>[2x]AGQQQPLPVPPLLESRRGQPLFMTVQRAHWSFTPGTRASVWGINGRYLGPTIRVWKGDDVKLIYSNRLTENVSMTVAGLQVPGPLMGGPARMMSPNADWAPVLPIRQNAATLWYHANTPNRTAQQVYNGLAGMWLVEDEVSKSLPIPNHYGVDDFPVIIQDKRLDNFGTPEYNEPGSGGFVGDTLLVNGVQSPYVEVSRGWVRLRLLNASNSRRYQLQMNDGRPLHVISGDQGFLPAPVSVKQLSLAPGERREILVDMSNGDEVSITCGEAASIVDRIRGFFEPSSILVSTLVLTLRPTGLLPLVTDSLPMRLLPTEIMAGSPIRSRDISLGDDPGINGQLWDVNRIDVTAQQGTWERWTVRADEPQAFHIEGVMFQIRNVNGAMPFPEDRGWKDTVWVDGQVELLVYFGQPSWAHFPFYFNSQTLEMADRGSIGQLLVNPVPRSHHHHHH

SufI is a water-soluble, periplasmic protein. The sequence of SufI shows that it is a member of the multicopper oxidase superfamily. The overall structure of SufI is very similar to that of CueO and contains three cupredoxin-like domains. Indeed, access to the region of the structure that forms the active site in multicopper oxidases is blocked in SufI by highly conserved residues. Together, these observations suggest that SufI is neither a copper-binding protein nor an enzyme.

The two molecules of each asymmetric unit are essentially the same within experimental error (rmsds over 408 and 406 Cα atoms of 1.1 and 0.9 Å for the orthorhombic and monoclinic crystals, respectively). Of the two data sets, the orthorhombic crystals diffracted to higher resolution (1.9 Å compared to 2.6 Å). The structure of SufI, determined here at a resolution of 1.9 Å by X-ray crystallography, confirms that the protein belongs to the multicopper oxidase family. No electron density was observed for the hexahistidine affinity tag, with the exception of the arginine residue of the affinity tag linker in chain A of the orthorhombic structure. The main areas of difference between the two crystal forms lie between residues 42–47, 55–66 and 326–334. Residues 42–47 are found in a loop that leads into the first domain, while residues 326–334 compose the long linker between domains 2 and 3. The electron density for both of these regions was poor and often missing entirely for the side chains. This suggests that these differences between the two crystal forms arise from flexibility of the molecule in these regions. Residues 55–66 are found in an extended loop in the first domain: a short alpha-helical segment is present in this loop in the orthorhombic form, which is unravelled in the monoclinic form.>MGLEKTVKEKLSFEGVGIHTGEYSKLIIHPEKEGTGIRFFKNGVYIPARHEFVVHTNHSTDLGFKGQRIKTVEHILSVLHLLEITNVTIEVIGNEIPILDGSGWEFYEAIRKNILNQNREIDYFVVEEPIIVEDEGRLIKAEPSDTLEVTYEGEFKNFLGRQKFTFVEGNEEEIVLARTFAFDWEIEHIKKVGLGKGGSLKNTLVLGKDKVYNPEGLRYENEPVRHKVFDLIGDLYLLGSPVKGKFYSFRGGHSLNVKLVKELAKKQKL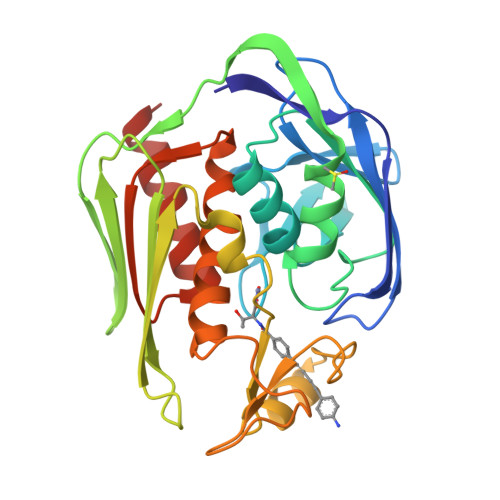TRDLP[2x]> GAHMNDIKQLLWNGELNVLVSIDPSFLMKGSPREIAVLRIRVPRETYLVNYMPLIWNKI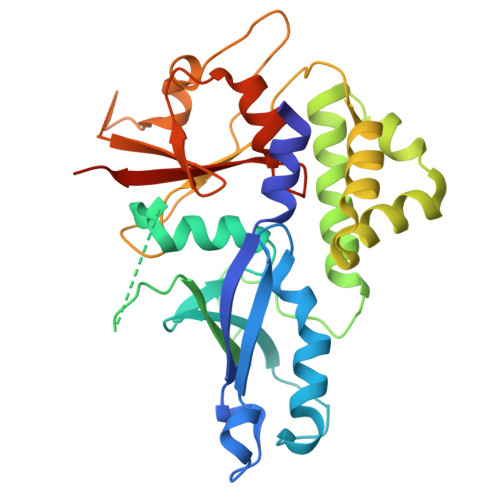KSFLSFDPLTDSEKYFWFEHNKTPIPWNYPVGVLFDCLAGKSATFTTSFENQVKDVLTFLRIHLVMGDSLPPTIIPIASSKTQAEKFWFHQWKQVCFILNGSSKAIMSLSVNEARKFWGSVITRNFQDFIEISNKISSSRPRHIPLIIQTSRTSGTFRISQPTISMTGVNPTLKDIEGDILDVKEGINGNDVMVICQGIEIPWHMLLYDLYSKLRSFDGFLYITLVPIKGGDKASSEL GUANOSINE | C10 H13 N5 O5 | 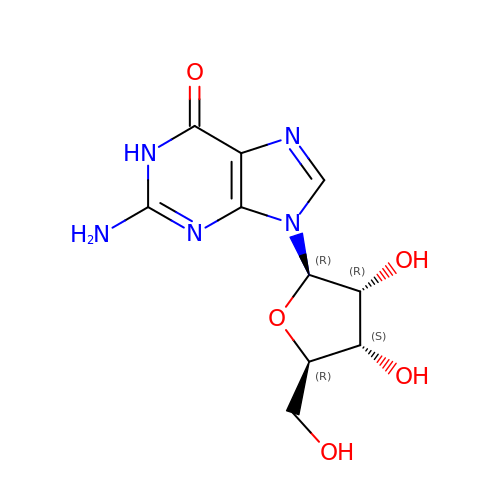NYHBQMYGNKIUIF-UUOKFMHZSA-N>[2x]DI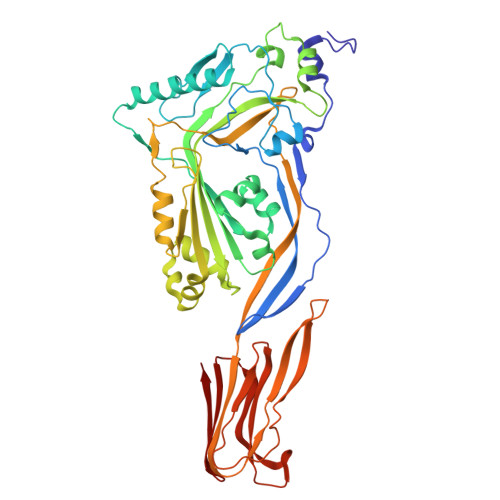TDKNQSIDSGISSLSYNRNEVLASNGDKIESFVPKEGKKAGNKFIVVERQKRSLTTSPVDISIIDSVNDRTYPGALQLADKALVENRPTILMVKRKPININIDLPGLKGENSIKVDDPTYGKVSGAIDELVSKWNEKYSSTHTLPARTQYSESMVYSKSQISSALNVNAKVLENSLGVDFNAVANNEKKVMILAYKQIFYTVSADLPKNPSDLFDDSVTFNDLKQKGVSNEAPPLMVSNVAYGRTIYVKLETTSSSKDVQAAFKALIKNTDIKNSQQYKDIYENSSFTAVVLGGDAQEHNKVVTKDFDEIRKVIKDNATFSTKNPAYPISYTSVFLKDNSVAAVHNKTDYIETTSTEYSKGKINLDHSGAYVAQFEVAWDEVSYDKEGNEVLTHKTWDGNYQDKTAHYSTVIPLEANARNIRIKARECTGLAWEWWRDVISEYDVPLTNNINVSIWGTTLYPGSSITYN>[4x]MAKRKIQRYVRKDGKCNVHHGNVRETYRYLTDIFTTLVDLKWRFNLLIFVMVYTVTWLFFGMIWWLIAYIRGDMDHIEDPSWTPCVTNLNGFVSAFLFSIETETTIGYGYRVITDKCPEGIILLLIQSVLGSIVNAFMVGCMFVKISQPKKRAETLVFSTHAVISMRDGKLCLMFRVGDLRNSHIVEAS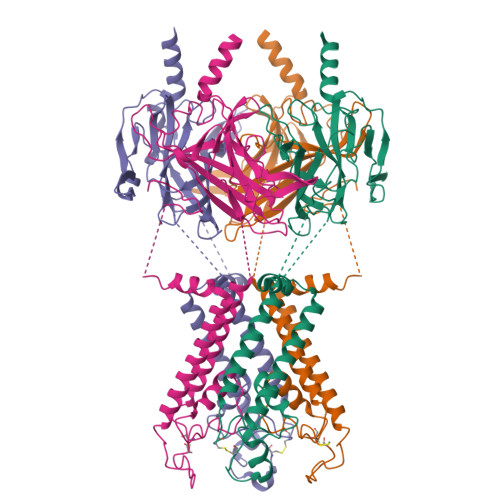IRAKLIKSKQTSEGEFIPLNQTDINVGYYTGDDRLFLVSPLIISHEINQQSPFWEISKAQLPKEELEIVVILEGMVEATGMTCQARSSYITSEILWGYRFTPVLTLEDGFYEVDYNSFHETYETSTPSLSAKELAELANRAESNSLEVLFQ> MRLTDAVNVTLEALG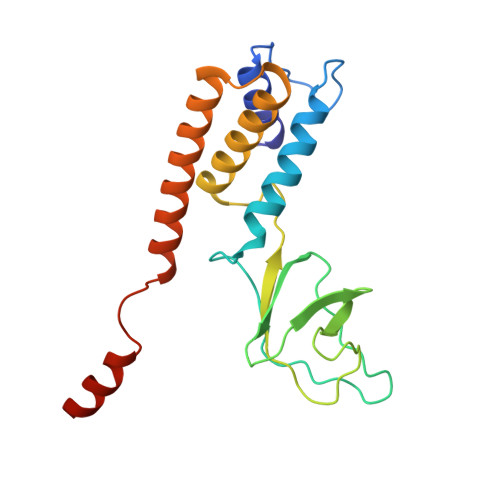ESRIVDINTSNPSAGLARAALDRTRRGVLSTGWWFNTIIREVTPTPNPGQIKVPWNQLSMYGLDGTKYGERDGVLYNLVDQTKVFSDTVHLKVVIDIDFEDLPEHMAMWVANATAAQVYLNDLGADGNYKSLLGIAAEYEAMNMREHLRNQRYSTSRTHAARKIRSGFFR> QIASDVEAPPP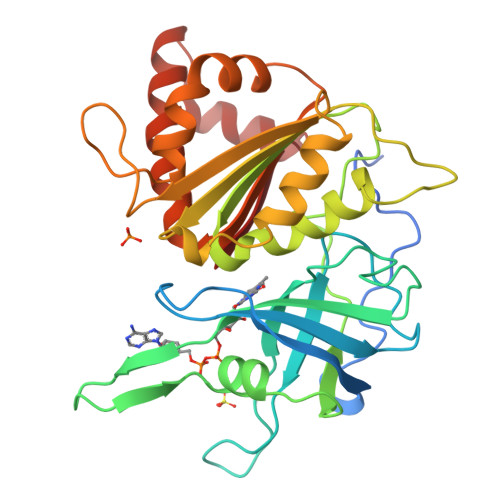APAKVEKHSKKMEEGITVNKFKPKTPYVGRCLLNTKITGDDAPGETWHMVFSHEGEIPYREGQSVGVIPDGEDKNGKPHKLRLYSIASSALGDFGDAKSVSLCVKRLIYTNDAGETIKGVCSNFLCDLKPGAEVKLTGPVGKEMLMPKDPNATIIMLGTGTGIAPFRSFLWKMFFEKHDDYKFNGLAWLFLGVPTSSSLLYKEEFEKMKEKAPDNFRLDFAVSREQTNEKGEKMYIQTRMAQYAVELWEMLKKDNTYFYMCGLKGMEKGIDDIMVSLAAAEGIDWIEYKRQLKKAEQWNVAVY Using X-ray crystallography, we show that the ciliopathy-associated centriolar protein CEP120 contains three C2 domains. CEP120, for example, plays a key role in the duplication, elongation, and maturation of centrioles, which in principle could impact the production of a functional basal body (Comartin et al., 2013, Lin et al., 2013, Mahjoub et al., 2010, Wu et al., 2014). All three C2 domains of CEP120 (C2A, C2B, and C2C) adopt the PLC δ1-like topology II and are structurally similar to each other (root-mean-square deviation [RMSD], 2.4–2.6 Å), with major differences found mainly in their loop length. Thus, the CEP120 C2 domains probably play a role as protein-protein interaction modules.

While the linker between C2A and C2B is short, the linker between C2B and C2C is ∼100 residues long and enriched with proline and charged residues but largely non-conserved and without predicted secondary structure elements. Our structures revealed neither complexed Ca2+ nor potential Ca2+-coordinating top loop residues or cationic β-grooves. Prime candidates for interaction interfaces in these domains are the regions defined by strands 3 and 4 at the edges of their β sandwich that constitute their most conserved parts.

>[3x]GPCGASEVVTSGQKIAVPAASHHFCFSVDLRSVHDLELSFPVNCILRYSYPFFGSAAPIMTNPPVEVRKNMEVFLPQSYCAFDFATMPHQLQDTFLRIPLLVELWHKDKMSKDLLLGVARIQLSNILSSEKTRFLGANGEQCWRQTYSESVPVIAAQGSNNRILDLSYTMTLEDYGLVKMREIFVSESSQGVPAVDQKPSS> ACDYTCGSNCYSSSDVSTAQAAGYKLHEDGETVGSNSYPHKYNNYEGFDFSVSSPYYEWPILSSGDVYSGGSPGADRVVFNENNQLAGVITHTGASGNNFVECT

To provide easy-to-use automated NCS restraints, it was decided to adopt a different approach that uses interatomic distances rather than structural superposition, extending the ideas used in the SHELX program. The restraints encourage NCS-related chains to have similar local structure, but differences are allowed to occur at a fixed cost. The restraints can also be used for another commonly encountered case of molecular similarity, namely that to a separate already determined structure that remains fixed during the refinement of the structure being refined.

Lenz et al. published the structure of ribonuclease T1 (RNAse T1) with the nucleotide guanosine-3′,5′-bisphosphate (pGp) bound. The structure was determined from an in­complete (90%) 3.2 Å resolution room-temperature data set collected on a four-circle diffractometer with a sealed-tube source. The same group later determined the structure of RNAse T1 with pGp bound at a much higher (1.8 Å) resolution. The pGp ligand-binding position differed from the previous low-resolution result, particularly in the positioning of the guanine ring. In addition, a phosphate anion was found to be bound in the catalytic site that had not been observed in the low-resolution structure. Accordingly, it was decided to re-solve RNAse T1–pGp. Positioning the pGp ligand with rhofit and subsequent refinement (with target LSSR) strengthened clear density for a separate tetrahedral anion in the catalytic site. Following Lenz et al. this was modelled as a phosphate. The pGp ligand conformation, its binding contacts and the positioning of the phosphate anion in the catalytic site are consistent with those described by Lenz et al. for the same complex solved at 1.8 Å resolution (see Supplementary Material1). It can be concluded that BUSTER ML refinement with target LSSR allows the most important features of the pGp T1 RNAse complex to be found from low-resolution data.Enzyme rhodopsins comprise the N-terminal rhodopsin domain and C-terminal enzyme domain, connected by a linker, and function as light-activated enzymes. Rh-PDE derived from Salpingoeca rosetta (SrRh-PDE) was first identified and exhibits light-dependent hydrolytic activity for both of cAMP and cGMP, whereas it lacks pump or channel activity. SrRh-PDE consists of the long N-terminal region, transmembrane domain (TMD), including the rhodopsin domain, C-terminal PDE domain, and 76-residue linker region connecting the TMD and PDE domain. Here, we present crystal structures of SrRh-PDE–TMD with and without the linker region, at 3.5 and 2.6 Å resolutions, respectively.

Thus, we expressed, purified and crystallized the TMD of Rh-PDE (Rh-PDE–TMD, residues 33–316). The structure was determined at 2.6 Å resolution by molecular replacement, using the structure of bacteriorhodopsin (BR, PDB ID: 1M0M22). The crystallographic asymmetric unit contained two molecules (mol A and mol B). In the Rh-PDE–TMD structure, the two protomers in the asymmetric unit form a dimer. The interfacial interactions occur in the intracellular halves of TM1 and TM7 of each molecule, whereas two monoolein molecules fill the dimer interface at the extracellular half. TM0 exists on the exterior of the rhodopsin domain, and is located between TM2 and TM3. Trp63 in TM0 hydrogen bonds with Ser136 in TM2, and the other residues form extensive hydrophobic interactions with TM2 and TM3. Lys296 at TM7 forms a covalent bond with a retinal-Schiff base (RSB) of all-trans retinal (ATR), as in the other microbial rhodopsins. In the Rh-PDE structure, Asp292 directly hydrogen bonds with the RSB, and the protonated Glu164 directly hydrogen bonds with Asp292. Moreover, there is no water molecule around the counterion in the current structure.

>[2x]MGRGKRRAKTRNIAIASTKEVQWQGIFMIIVWLCVMGSLIFFANPEASRRVFAKFSHLQSFYGATSVAFAFATGLDILAYVNAVSDEKRVLSGILAYVDGVACISYLSMATLNLYFLVDSTQGNPVWLMRYAEWIITCPTLLYWCGLASRADRSSVSDIATADALLLAGGALSSILPSWPAFFVFAGSFATYIYVMLHMWGMFGKAMQPDFQPPPPLPRHALHLLRCEIVMSWSIFPLVEFLRRQGYIDFQVGEAMNCVADYAAKVGLAMIMVNCNLEQINALRVENLYFQ>[4x]GPGSQDVNVVYKSALSLYDVSLALLVAQKSQMDPREYLPFLQELQDNEPLRRKFLIDDYLGNYEKALEHLSEIDKDGNVSEEVIDYVESHDLYKHGLALYRYDSEKQNVIYNIYAKHLSSNQMYTDAAVAYEMLGKLKEAMGAYQSAKRWREAMSIAVQKFPEEVESVAEELISSLTFEHRYVDAADIQLEYLDNVKEAVALYCKAYRYDIA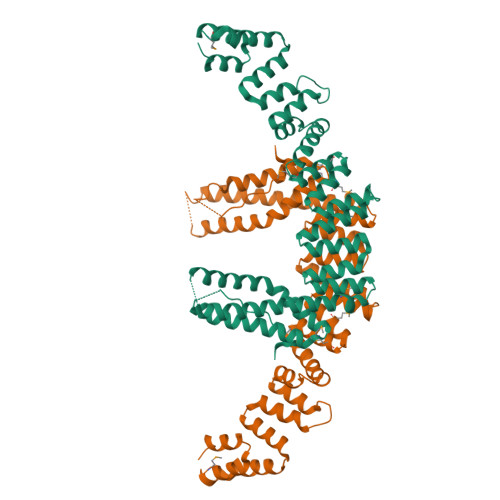SLVAIKAKKDELLEEVVDPGLGEGFGIIAELLADCKGQINSQLRRLRELRAKKEENPYAFYGQETEQADDVSVAPSETSTQESFFTRYTGKTGGTAKTGASRRTAKNKRREERKRARGKKGTIYEEEYLVQSVGRLIERLNQTKPDAVRVVEGLCRRNMREQAHQIQKNFVEVLDLLKANVKEIYSISEKDRERVNENGEVYYIPEIPVPEIHDFPKSHIVDF> KTVIKNETGTISISQLNKNVWVHTELGSFNGEAVPSNGLVLNTSKGLVLVDSSWDDKL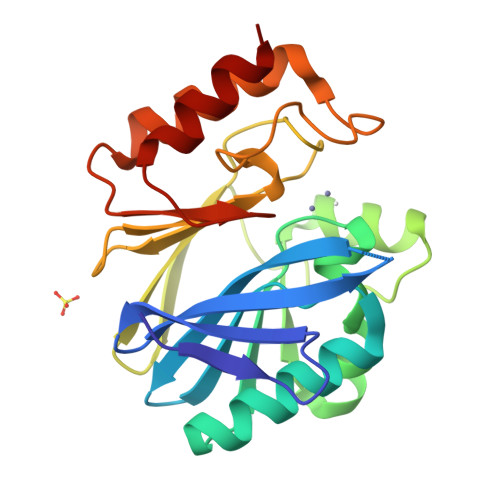TKELIEMVEKKFQKRVTDVIITHAHADRIGGIKTLKERGIKAHSTALTAELAKKNGYEEPLGDLQTVTNLKFGNMKVETFYPGKGHTEDNIVVWLPQYNILVGGCLVKSTSAKDLGNVADAYVNEWSTSIENVLKRYRNINAVVPGHGEVGDKGLLLHTLDLLK WbdD is a bifunctional kinase/methyltransferase that is responsible for regulation of lipopolysaccharide O antigen polysaccharide chain length in Escherichia coli serotype O9a. WbdD is a soluble protein that controls the length of some lipopolysaccharide O-antigen polysaccharides that are synthesized in an ABC-transporter-dependent pathway. WbdD from Escherichia coli O9a contains two enzymatic domains: a methyltransferase (MTase) domain and a kinase domain. WbdD stops polymerization of the chain by phosphorylating and then methylating the phosphate on the terminal sugar.

We therefore designed, cloned and expressed a new construct, WbdD556 (residues 1–556), that was purified in the same way as WbdD600. We found a single native crystal that diffracted to better than 3.0 Å resolution (crystal category A), although there was no obvious visual indication as to why and this could not be reproduced. This crystal grew from the ammonium sulfate-based condition, but was harvested more than six months after the plate had been set up. During the intervening time, approximately half of the volume of the reservoir solution had evaporated, leaving a much higher (∼2 M) concentration of ammonium sulfate. By comparing the unit-cell parameters of the different crystal categories (A, B, C and D), we found that the decrease in length of the cubic unit-cell axis from 185 Å in crystal category D to 167 Å in crystal category A generally correlated with resolution. Data from a serendipitously found single native crystal that diffracted to 3.0 Å resolution were non-isomorphous with a lower (3.5 Å) resolution selenomethionine data set. Here, a strategy for improving poor (3.5 Å resolution) initial phases by density modification and cross-crystal averaging with an additional 4.2 Å resolution data set to build a crude model of WbdD is desribed. Using this crude model as a mask to cut out the 3.5 Å resolution electron density yielded a successful molecular-replacement solution of the 3.0 Å resolution data set. The resulting map was used to build a complete model of WbdD. The best diffracting crystals (which also belonged to space group I23) had a unit-cell parameter of 158 Å, which is again considerably shorter than the 167 Å unit-cell parameter of the native crystal that was used to solve the initial structure.

> MHHHHHHENLYFQGTKDLNTLVSELPEIYQTIFGHPEWDGDAARDCNQRLDLITEQYDNLSRALGRPLNVLDLGCAQGFFSLSLASKGATIVGIDFQQENINVCRALAEENPDFAAEFRVGRIEEVIAALEEGEFDLAIGLSVFHHIVHLHGIDEVKRLLSRLADVTQAVILELAVKEEPFYWGVSQPDDPRELIEQCAFYRLIGEFDTHLSPVPRPMYLVSNHRVLINDFNQPFQHWQNQPYAGAGLAHKRSRRYFFGEDYVCKFFYYDMPHGILTAEESQRNKYELHNEIKFLTQPPAGFDAPAVLAHGENAQSGWLVMEKLPGRLLSDMLAAGEEIDREKILGSLLRSLAALEKQGFWHDDVRPWNVMVDARQHARLIDFGSIVTTPQDCSWPTNLVQSFFVFVNELFAENKSWNGFWRSAPVHPFNLPQPWSNWLYAVWQEPVERWNFVLLLALFEKKAKLPSAEQQRGATEQWIIAQETVLLELQSRVRNESAGSEALRGQIHTLEQQMAQLQSAQDAFVEKAQQQVEVSHELTWLGENMEQLAALLQTAQAHAQADVQPELPP>STAGKVIKCKAAVLWEEKKPFSIEEVEVAPPKAHEVRIKMVATGICRSDDQVVSGTLVTPLPVIAGHEAAGIVESIGEGVTTVRPGDKVIPLFTPQCGKCRVCKHPEGNFCLKNDLSMPRGTMQDGTSRFTCRGKPIHHFLGTSTFSQYTVVDEISVAKIDAASPLEKVCLIGCGFSTGYGSAVKVAKVTQGSTCAVFGLGGVGLSVIMGCKAAGAARIIGVDINKDRFAKAKEVGATECVNPQDYKKPIQEVLTEMSNGGVDFSFEVIGRLDTMVTALSCCQEAYGVSVIVGVPPDSQNLSMNPMLLLSGRTWKGAIFGGFKSKDSVPKLVADFMAKKFALDPLITHVLPFEKINEGFDLLRSGESI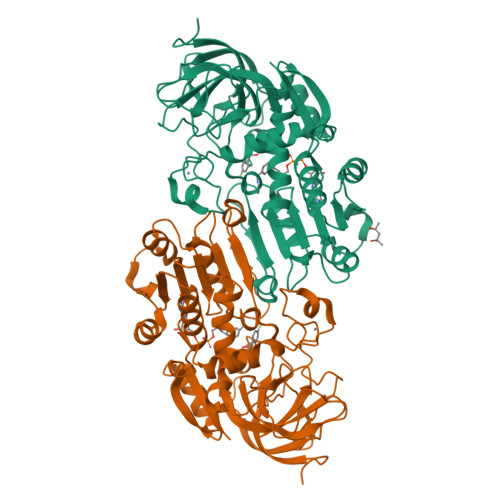RTILTF[2x]>SMAAAEGPVGDGELWQTWLPNHVVFLRLREGLKNQSPTEAEKPASSSLPSSPPPQLLTRNVVFGLGGELFLWDGEDSSFLVVRLRGPSGGGEEPALSQYQRLLCINPPLFEIYQVLLSPTQHHVALIGIKGLMVLELPKRWGKNSEFEGGKSTVNCSTTPVAERFFTSSTSLTLKHAAWYPSEILDPHVVLLTSDNVIRIYSLREPQTPTNVIILSEAEEESLVLNKGRAYTASLGETAVAFDFGPLAAVPKTLFGQNGKDEVVAYPLYILYENGETFLTYISLLHSPGNIGKLLGPLPMHPAAEDNYGYDACAVLCLPCVPNILVIATESGMLYHCVVLEGEEEDDHTSEKSWDSRIDLIPSLYVFECVELELALKLASGEDDPFDSDFSCPVKLHRDPKCPSRYHCTHEAGVHSVGLTWIHKLHKFLGSDEEDKDSLQELSTEQKCFVEHILCTKPLPCRQPAPIRGFWIVPDILGPTMICITSTYECLIWP[2x];>GPHMAGIILTKVGYYTIPSMDDLAKITNEKGECIVSDFTIGRKGYGSIYFEGDVNLTNLNLDDIVHIRRKEVVVYLDDNQKPPVGEGLNRKAEVTLDGVWPTDKTSRCLIKSPDRLADINYEGRLEAVSRKQGAQFKEYRPET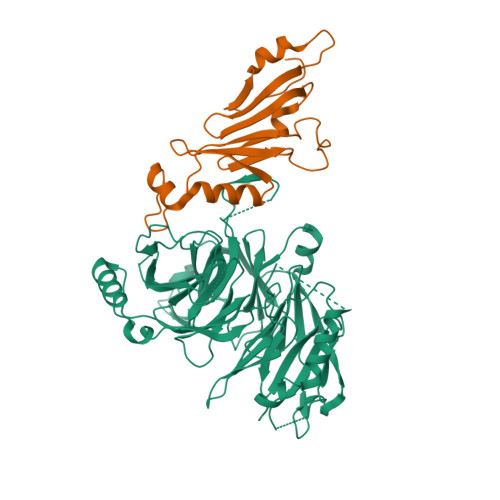GSWVFKVSHF[2x]> MAQRQFFGLTYNFYGQPAPLFDLNDLQELAGCYARPWTSRFSHLAISTGSLPVWSARYPSVASRNIVVNTLLGAHLNPFAGGQITSHQGITWRDPVLSSLAPVPAIQPPPVWAVAENVLLDSNNYPTYVLNLSSMWPINQDVHIMTMWALSDQGPIYHLEVPVDPMPAATTAALMAYTGVPIAHLAQTAYRFAGQLPQSPDSTMV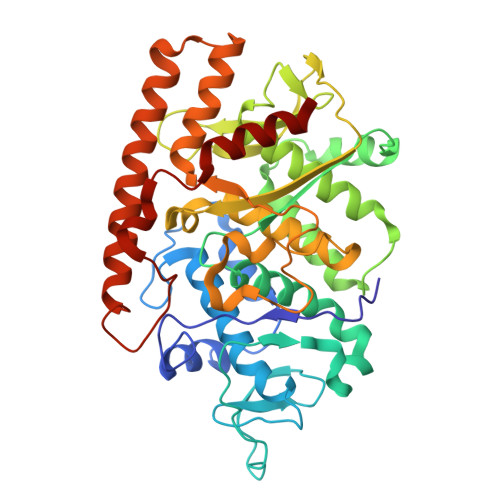STIRWLSAIWFGSLTGRLNRSRTCNGFYFEFAKPALNPDQAVLKWNDGARAAPPAAAQSSYIRCISPHWQHQIVEVAGALMSQSVTAVTGLPALIDEATLPAWSQGVANLTGNGQGVVPCLDYNPVPMAAARHLQWRQDGLITAAQEAQLNNDYTAYALTIERHLTAMLVANPIAAGRMPIQPFNAADFGQAGQTAAAVALAQAMFV>GPMANSSVELRVLEARPEDVGRKIVRMDKQTRARLGVSVGDYVEVKKVDRSVVARVLPARPEDVGRGIVRMDKYLRAALGVSVGDYVE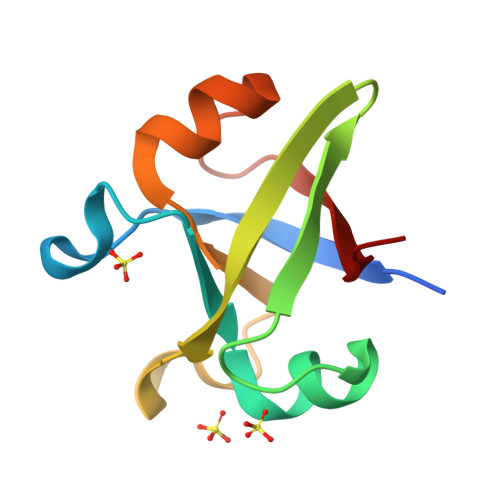VKKVE[3x]> VTIDNIQKTVAEYYKIKVADLLSKRRSRSVARPRQMAMALAKELTNHSLPEIGDAF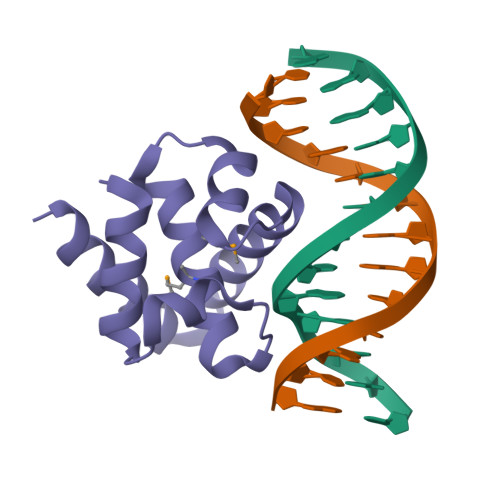GGRDHTTVLHACRKIEQLREESHDIKEDFSNLIRTLSS> SLEEGEASSTTSPTEETTQKLTVSHIEGYECQPIFLNVL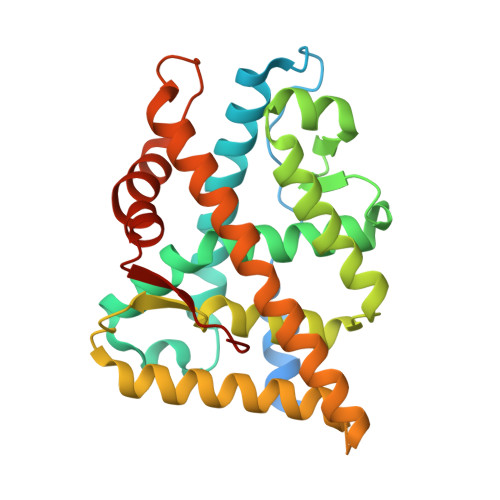EAIEPGVVCAGHDNNQPDSFAALLSSLNELGERQLVHVVKWAKALPGFRNLHVDDQMAVIQYSWMGLMVFAMGWRSFTNVNSRMLYFAPDLVFNEYRMHKSRMYSQCVRMRHLSQEFGWLQITPQEFLCMKALLLFSIIPVDGLKNQKFFDELRMNYIKELDRIIACKRKNPTSCSRRFYQLTKLLDSVQPIARELHQFTFDLLIKSHMVSVDFPEMMAEIISVQVPKILSGKVKPIYFHTQEG>[8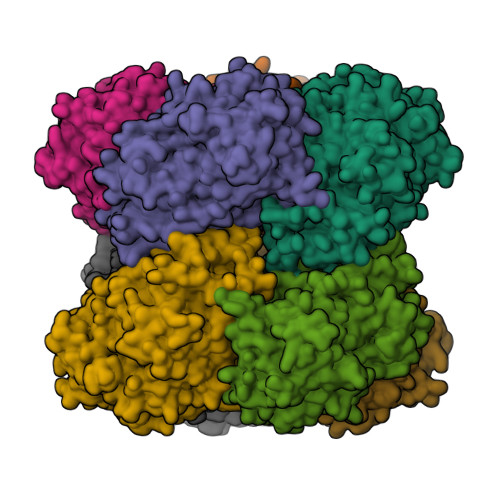x]MGHPEEVDVIVCGGGPAGCVVAGRLAYADPTLKVMLIEGGANNRDDPWVYRPGIYVRNMQRNGINDKATFYTDTMASSYLRGRRSIVPCANILGGGSSINSQMYTRASASDWDDFKTEGWTCKDLLPLMKRLENYQKPCNNDTHGYDGPIAISNGGQIMPVAQDFLRAAHAIGVPYSDDIQDLTTAHGAEIWAKYINRHTGRRSDAATAYVHSVMDVQDNLFLRCNARVSRVLFDDNNKAVGVAYVPSRNRTHGGKLHETIVKARKMVVLSSGTLGTPQILERSGVGNGELLRQLGIKIVSDLPGVGEQYQDHYTTLSIYRVSNESITTDDFLRGVKDVQRELFTEWEVSPEKARLSSNAIDAGFKIRPTEEELKEMGPEFNELWNRYFKDKPDKPVMFGSIVAGAYADHTLLPPGKYITMFQYLEYPASRGKIHIKSQNPYVEPFFDSGFMNNKADFAPIRWSYKKTREVARRMDAFRGELTSHHPRFHPASPAACKDIDIETAKQIYPDGLTVGIHMGSWHQPSEPYKHDKVIEDIPYTEEDDKAIDDWVADHVETTWHSLGTCAMKPREQGGVVDKRLNVYGTQNLKCVDLSICPDNLGTNTYSSALLVGEKGADLIAEELGLKIKTPHAPVPHAPVPTGRPATQQVR>MGAHSKEMAPLMGKRTTAPGGNPVVLTEKRPADLTPTKKSAHFFLEIEGFEPNPTVTKTSPPIFSKPMDSNIRQCLSGNCDDMDSPQSPQDDVTETPSNPNSPSANLAKEEQRQKKKRLKKRIFAAVSEGCVEELRELLQDLQDLCRRRRGLDVPDFLMHKLTASDTGKTCLMKALLNINPNTKEIVRILLAFAEENDILDRFINAEYTEEAYEGQTALNIAIERRQGDITAVLIAAGADVNAHAKGVFFNPKYQHEGFYFGETPLALAACTNQPEIVQLLMENEQTDITSQDSRGNNILHALVTVAEDFKTQNDFVKRMYDMILLRSGNWELETMRNNDGLTPLQLAAKMGKAEILKYILSREIKEKPLRSLSRKFTDWAYGPVSSSLYDLTNVDTTTDNSVLEIIVYNTNIDNRHEMLTLEPLHTLLHTKWKKFAKYMFFLSFCFYFFYNITLTLVSYYRPREDEDLPHPLALTHKMSWLQLLGRMFVLIWATCISVKEGIAIFLLRPSDLQSILSDAWFHFVFFVQAVLVILSVFLYLFAYKEYLACLVLAMALGWANMLYYTRGFQSMGMYSVMIQKVILHDVLKFLFVYILFLLGFGVALASLIEKCSKDKKDCSSYGSFSDAVLELFKLTIGLGDLNIQQNSTYPILFLFLLI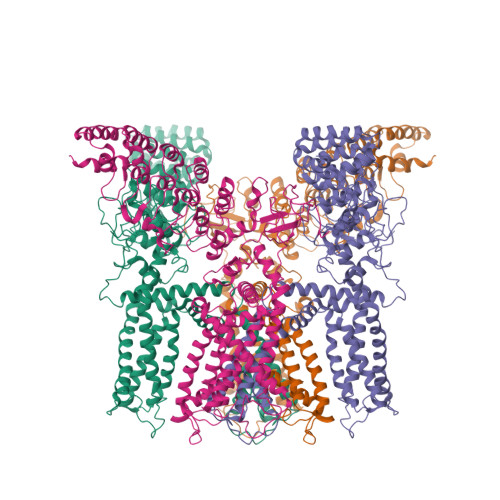TYVILTFVLLLNMLIALMGETVENVSKESERIWRLQRARTILEFEKMLPEWLRSRFRMGELCKVADEDFRLCLRINEVKWTEWKTHVSFLNEDPGPIRRTADLNKIQDSSRSNSKTTLYAFDELDEFPETSV[4x]> KPEPTDEEWELIKTVTEAHVATNAQGSHWKQKRKFLPEDIGQAPIVNAPEGGKVDLEAFSHFTKIITPAITRVVDFAKKLPMFCELPCEDQIILLKGCCMEIMSLRAAVRYDPESETLTLNGEMAVTRGQLKNGGLGVVSDAIFDLGMSLSSFNLDDTEVALLQAVLLMSSDRPGLACVERIEKYQDSFLLAFEHYINYRKHHVTHFWPKLLMKVTDLRMIGACHASWFLHMKVECPT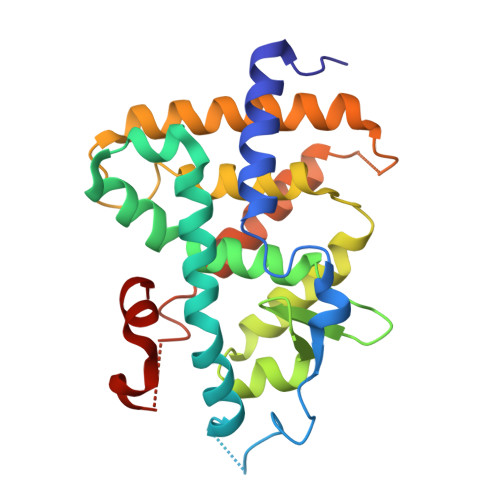ELFPPLFLEVFE> XVD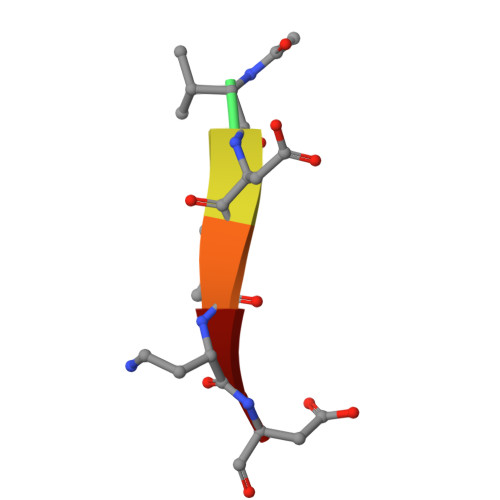VAD>[2x]MPLSAFSPPLPCDPARSHPTPEFPSSLQDYCEIRGIQS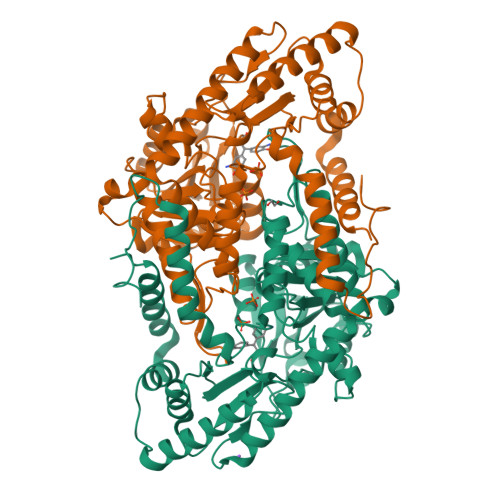QPPARRDPTMDWLASLRSQIKPYRDRFPSHARLPRAGLPRAEILAEIAAMGAAESPAWRDGYASGAVYHGDEHHIAFLNEVYALQSQSNPLHPDLWPSTAKFEAEVVAMTAHMLGGDAAGGTVCGTVTSGGTESLLLAMKTYRDWARATKGITAPEAVVPVSAHAAFDKAAQYFGIKLVRTPLDADYRADVAAMREAITPNTVVVAGSAPGYPHGVVDPIPEIAALAAEHGIGCHVDACLGGFILPWAERLGYPVPPFDFRLEGVTSVSADTHKYGYGAKGTSVILYRRPDLLHYQYFIAADWPGGLYFSPTFAGSRPGALSATAWAAMLSLGEEGYLDATRRILQAADRLKAGVRAIPSLKILGDPLWVIAVASDELNIYQVMEEMAGRGWRLNGLHRPPAFHVALTLRHTEPGVVDRFLADLQDAVAQVRAHPEKATGMAPVYGMAAAAPPELVRQVLTGFIDLLYEVHHHHHH> SLRKQRFMQFSSLEHEGEYYMTPRDFLFSVMFEQMERKTSVKKLTKKDIEDTLSGIQTAGCGSTFFRDLGDKGLISYTEYLFLLTILTKPHSGFHVAFKMLDTDGNEMIEKREFFKLQKIISKQDDLMTVKTNETGYQEAIVKEPEINTTLQMRFFGKRGQRKLHY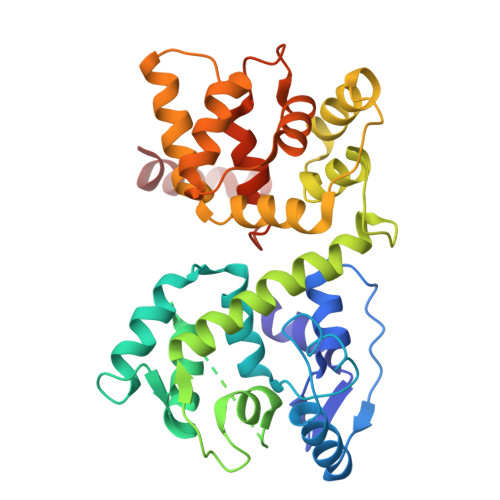KEFRRFMENLQTEIQEMEFLQFSKGLSFMRKEDFAEWLLFFTNTENKDIYWKNVREKLSAGESISLDEFKSFCHFTTHLEDFAIAMQMFSLAHRPVRLAEFKRAVKVATGQELSNNILDTVFKIFDLDGDECLSHEEFLGVLKNRMHRGLWVPQHQSIQEYWKCVKKES>[2x]GPLGSTIITSLQRKEGHSLGFSITGGFKQADGQYS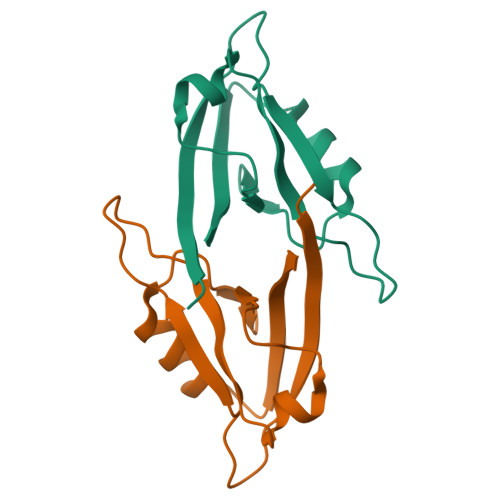GIYISKIAKDSIAAVDGKLSAGDILLKINDESMTNVPHSRAVQMLRSEGKIITIVASRQQ4-piperidin-4-yloxypyridine-2-carboxamide | C11 H15 N3 O2 | 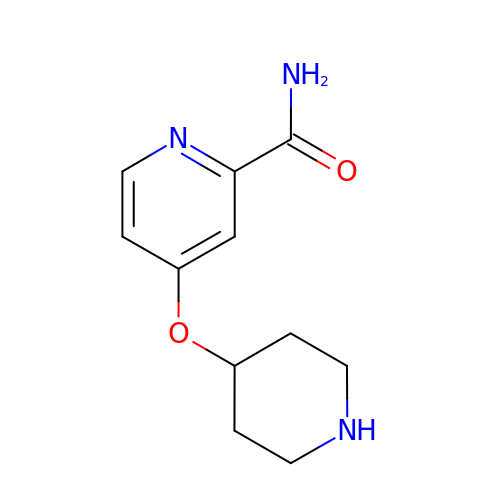NMMFHPWVBDVMFL-UHFFFAOYSA-N For this bacterium, Feo is the primary system that transports Fe2+ into the cytosol. FeoA and FeoC are known to be small (ca. 7–10 kDa) cytosolic proteins, while FeoB is a large (ca. 80–100 kDa) polytopic transmembrane protein that contains an N-terminal soluble G-protein-like domain termed NFeoB. The status of GTP and GDP bound to the NFeoB region is hypothesized to control the opening and closing of the FeoB pore and therefore the translocation of Fe2+ into the bacterial cytosol.

To prepare the VcNFeoB NTPase domain for crystallization trials, we overproduced in Escherichia coli a previously designed construct that encodes for a non-cleavable (His)6-tagged version of the protein (i.e., VcNFeoB(His)6). First, regarding AEX, we monitored the 260 nm/280 nm ratio through the entire chromatography process, and noted a normal value of ≈0.6, indicating that VcNFeoB(His)6 does not co-purify with nucleotide, unlike previous reports of E. coli NFeoB overproduced in E. coli. Second, SEC of either crudely purified VcNFeoB(His)6 (IMAC only) or polished VcNFeoB(His)6 (after SEC) showed only the presence of a dominant monomeric species in solution, consistent with our previous in vitro studies on Feo proteins (from V. cholerae and others) recombinantly produced in E. coli. In order to characterize the three-dimensional structure of the VcNFeoB NTPase domain, we sought to crystallize the VcNFeoB(His)6 protein. Crystals of the apo domain were generated and ultimately diffracted to a modest 3.7 Å resolution in the P1 space group consistent with 8 molecules (dimer of tetramers) in the asymmetric unit (ASU). This oligomerization is likely crystallization-induced based on our in-solution studies. We solved this structure by using molecular replacement coupled with model building and restrained refinement approaches (Rw/Rf = 0.210/0.268), and an analysis of the crystal contacts suggested that the (His)6 tag may have impacted the crystal quality.

>[8x]MKYQVLTVGNPNSGKTTLFNGLTGAKQQVGNWAGVTVEKKTGSFVHAGDEFSLTDLPGIYALDSGNDSNSIDESIASRAVLTHPADVIINVVDATCLERSLYMTLQLRELRRPMIVVLNKMDALKRERVHLDLKQLEAFLGCPVLALSANNKEQVRRFKEKLHKLLVQGIALKQIELHYGAEFESLIHELEPMFAEQAVSARALAIRALENDRLVINGLKEAERQNVEQRQHECQVDIDLLVANVRYTYLHELCTHVRRTEGKLSHKFTEKAKLAAALEHHHHHH> MMFGRFTERAQKVLALAQEEALRLGHNNIGTEHILLGLVREGEGIAAKALQALGLGSEKIQKEVESLIGRGQEMS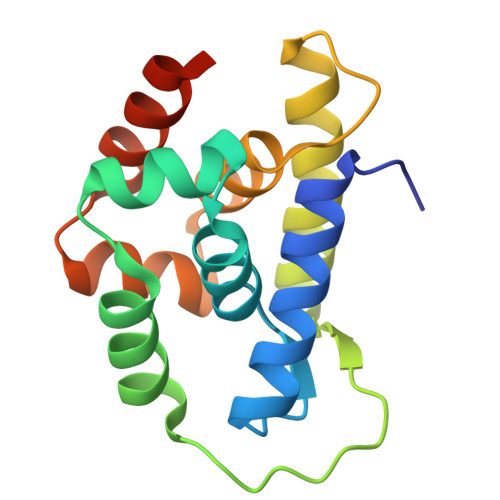QTIHYTPRAKKVIELSMDEARKLGHSYVGTEHILLGLIREGEGVAARVLNNLGVSLNKARQQVLQLLGSNETGS> ALQCFCHLCTKDNFTCVTDGLCFVSVTETTDKVIHNSMCIAEIDLIPRDRPFVCAPSSKTG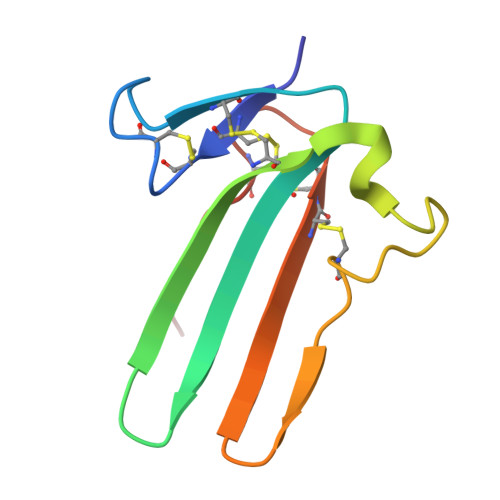SVTTTYCCNQDHCNKIELP> GVGISTGTFNNQTEFKFLENGWVEITANSSRLVHLNMPESENYRRVVVNNMDKTAVDGNMALDDIHAEIVTPWSLVDANAWGVWFNPGDWQLIVNTMSELHLVSFEQEIFNVVLKTVSESATQPPTKVYNNDLTASLMVALDSNNTMPFTPAAMRSETLGFYPWKPTIPTPWRYYFQWDRTLIPS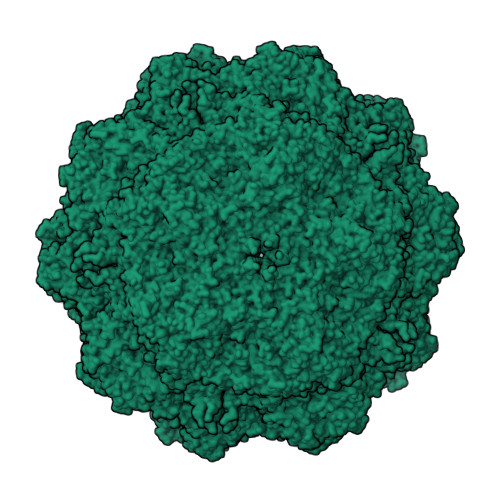HTGTSGTPTNIYHGTDPDDVQFYTIENSVPVHLLRTGDEFATGTFFFDCKPCRLTHTWQTNRALGLPPFLNSLPQSEGATNFGDIGVQQDKRRGVTQMGNTNYITEATIMRPAEVGYSAPYYSFEASTQGPFKTPIAAGRGGAQTDENQAADGNPRYAFGRQHGKKTTTTGETPERFTYIAHQDTGRYPEGDWIQNINFNLPVTNDNVLLPTDPIGGKTGINYTNIFNTYGPLTALNNVPPVYPNGQIWDKEFDTDLKPRLHVNAPFVCQNNCPGQLFVKVAPNLTNQYDPDASANMSRIVTYSDFWWKGKLVFKAKLRASHTWNPIQQMSINVDNQFNYVPSNIGGMKIVYEKSQLAPRKLY> MGKREYPSSAHFLVTLSL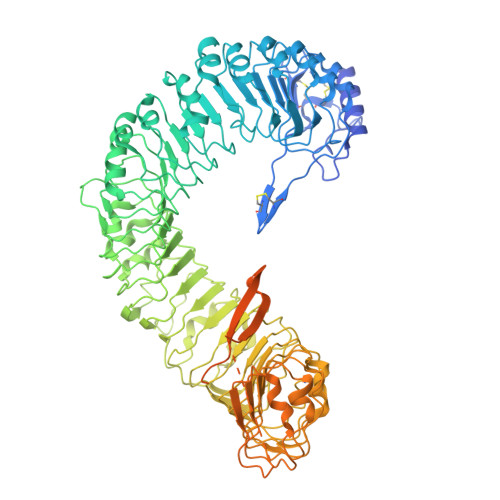LLLQAAFGLTLCIEKERDALLEFKRGLSDNFGQLSTWGDEEDKKECCKWKGIECNKTTGHVIVLDLHNAFTCSASACFAPRLTGKLSPSLLELEYLNFLDLSVNEFERSEIPRFICSFKRLEYLNLSSSFFSGLIPTQFKNLTSLRILDLGYNNLIVKDLTWLSHLSSLELLSLGGSDFQVKNWFQEITKLPLLKELDLSLCGLSKLVPSPAEIANSSLISLSVLHLCCNEFSSSAKYSWLFNFSTSLTSIDLSNNQLDGQIDDRFGNLMYLEHLNLANELNLKGGIPSSFGNLTRLRYLDMSNTRTYQWLPELFVRLSGSRKTLEVLGLNDNSMFGSLVDVTRFSALKRLYLQKNVLNGFFMERFGQVSSLEYLDLSDNQMRGPLPDLALFPSLRELHLGSNHFNGRIPQGIGKLSQLKILDVSSNRLEGLPESMGQLSNLESFDASYNVLKGTITESHLSNLSSLVDLDLSFNSLALKTSIDWLPPFQLQVINLPSCNLGPSFPKWLQSQNNYTVLDISLANISDALPSWFSGLPPDIKILNLSNNQISGRVSDLIENAYDYMVIDLSSNNFSGPLPLVPTNVQIFYLHKNQFFGSISSICKSTTGATSLDLSHNQFSGELPDCWMNATNLAVLNLAYNNFSGKLPQSLGSLTNLEALYMRQNSFSGMLPSLSQCQSLQILDLGGNKLTGRIPAWIGTDLLNLRILSLRFNKFYGSISPIICQLQFLQILDLSANGLAGKIPQCFNNFTLLHQENGLGEPMEFLVQGFYGKYPRHYSYLGNLLVQWKNQEAEYKNPLTYLKTIDLSSNKLVGGIPKEMAEMRGLKSLNLSRNDLNGSIIKGIGQMKMLESLDLSRNQLSGMIPKDLANLTFIGVLDLSNNHLSGRIPSSTQLQTFERSSYSGNAQLCGPPLQEC>[4x]MAEMLVKSKVKEFVKSVDPEMRVSPEFYDALEAEVKALVEKAIKRAQA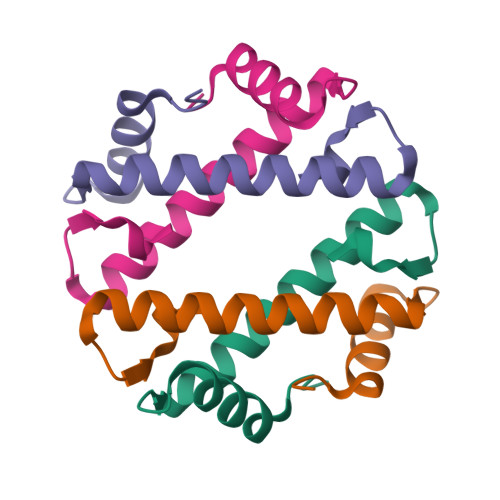EGRKTLYARHV> GSHMDLGAPQNPNAKAAGSRKIHFNWLPPSGKPMGYRVKYWIQG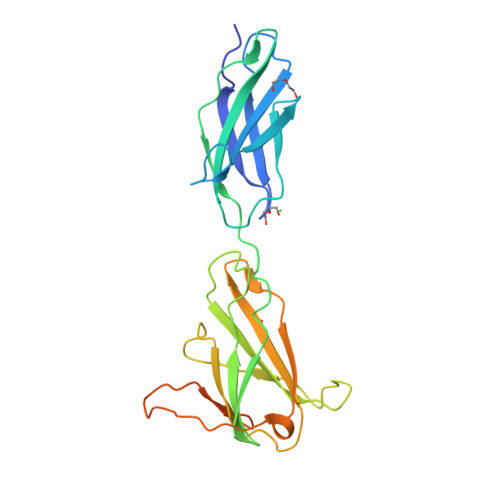DSESEAHLLDSKVPSVELTNLYPYCDYEMKVCAYGAQGEGPYSSLVSCRTHQEVPSEPGRLAFNVVSSTVTQLSWAEPAETNGEITAYEVCYGLVNDDNRPIGPMKKVLVDNPKNRMLLIENLRESQPYRYTVKARNGAGWGPEREAIINLATQPKRPMSIPIIPDIPIVDAQSGEDYDSFLMYSDDVLRSPSGSQRPSVSDDTE(2R)-2,5-diaminopentanoyl dihydrogen phosphate | C5 H13 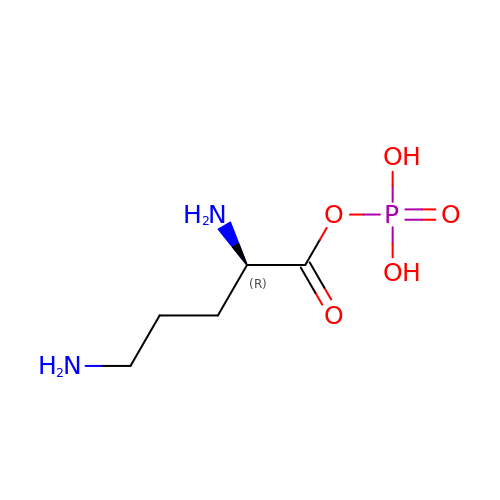N2 O5 P | MNDHJWIHMSHXOW-SCSAIBSYSA-N>GSPGTPEVKVASSEDVDLPCTAPWDPQVPYTVSWVKLLEGGEERMETPQEDHLRGQHYHQKGQNGSFDAPNERPYSLKIRNTTSSNSGTYRCTLQD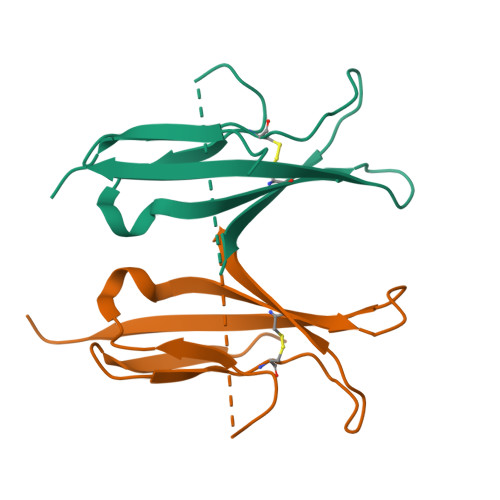PDGQRNLSGKVILRVTGSPA[2x]> AGIAAKLAKDREAAEGLGSHERAIKYLNQDYEALRNECLEAGTLFQDPSFPAIPSALGFKELGPYSSKTRGMRWKRPTEICADPQFIIGGATRTDICQGALGDCWLLAAIASLTLNEEILARVVPLNQSFQENYAGIFHFQFWQYGEWVEVVVDDRLPTKDGELLFVHSAEGSEFWSALLEKAYAKINGCYEALSGGATTEGFEDFTGGIAEWYELKKPPPNLFKIIQKALQKGSLLGCSIDITSAADSEAITFQKLVKGHAYSVTGAEEVESNGSLQKLIRIRNPWGEVEWTGRWNDNCPSWNTIDPEERERLTRRHEDGEFWMSFSDFLRHYSRLEICNLTPDTLTSDTYKKWKLTKMDGNWRRGSTAGGCRNYPNTFWMNPQYLIKLEEEDEDEEDGESGCTFLVGLIQKHRRRQRKMGEDMHTIGFGIYEVPEELSGQTNIHLSKNFFLTNRARERSDTFINLREVLNRFKLPPGEYILVPSTFEPNKDGDFCIRVFSEKKADYQAVDDEIEANLEEFDISEDDIDDGVRRLFAQLAGEDAEISAFELQTILRRVLAKRQDIKSDGFSIETCKIMVDMLDSDGSGKLGLKEFYILWTKIQKYQKIYREIDVDRSGTMNSYEM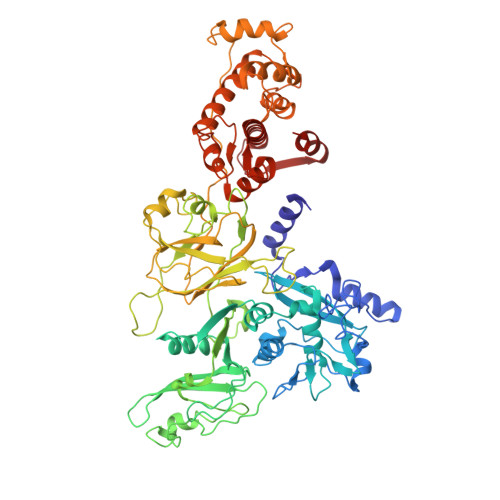RKALEEAGFKMPCQLHQVIVARFADDQLIIDFDNFVRCLVRLETLFKIFKQLDPENTGTIELDLISWLCFSVL The heterodimeric complex IrtAB has been identified as being responsible for the import of the two iron-loaded siderophores (Fe3+-MBT and Fe3+-cMBT) from the periplasmic space into the cytoplasm of Mtb and other mycobacteria. This protein complex is vital for the replication and viability of Mtb in macrophages, which reside in the lung alveoli. Like other ABC transporters, IrtAB contains two transmembrane domains (TMDs) and two nucleotide-binding domains (NBDs), with a single TMD and a single NBD in each of IrtA and IrtB. Interestingly, although IrtAB functions as an ABC importer, it adopts the canonical fold of type IV ABC exporters, which are normally responsible for the efflux of intracellular substrates such as the multidrug resistance protein, Sav1866.

To trap IrtAB in its ATP-bound state, the catalytic glutamate residues (Glu771 in IrtA and Glu495 in IrtB) were replaced by glutamine (IrtAB (E-Q)). By contrast, the SID-truncated IrtAB (E-Q) (IrtABΔSID (E-Q)) incubated with 10 mmol/L ATP-Mg2+ was suitable for cryo-EM and could be resolved at 3.1 Å resolution. Addition of ATP-Mg2+ resulted in an overall conformation that is substantially different from that of the ATP-free form. At the cytoplasmic side, the two NBDs of IrtA and IrtB form a “head-to-tail” dimer, characteristic of ABC transporters. Two ATP molecules are bound at the dimer interface, each of which is stabilized by an interaction between a Walker A motif in one NBD (IrtA or IrtB) and an ABC signature motif in the other NBD (IrtB or IrtA). Two magnesium ions are also observed, which ligand between the β- and γ-phosphates of ATP, a serine in the Walker A motif and the Q-loop glutamine, near the ABC signature motif. The TMHs of IrtAB do not split into two wings when ATP binds. As a result, the TMHs pack closely together to form an occluded amphipathic cavity with an approximate volume of ~4,600 Å3 (~2,700 Å3 in IrtA and ~1,900 Å3 in IrtB), which spans the entire thickness of the membrane and extends to the intracellular part of IrtAB. The marked difference between these two structures in the occluded state is that an additional unknown metal ion is observed in the cavity of IrtAB. However, the precise identity of the metal ion needs to be identified with more studies. This metal is bound to IrtA only and is liganded to three histidine residues (His356, His402, and His407), which are highly conserved across mycobacteria.

> MARGLQGVMLRSFGARDHTATVIETISIAPHFVRVRMVSPTLFQDAEAEPAAWLRFWFPDPNGSNTEFQRAYTISEADPAAGRFAVDVVLHDPAGPASSWARTVKPGATIAVMSLMGSSRFDVPEEQPAGYLLIGDSASIPGMNGIIETVPNDVPIEMYLEQHDDNDTLIPLAKHPRLRVRWVMRRDEKSLAEAIENRDWSDWYAWATPEAAALKCVRVRLRDEFGFPKSEIHAQAYWNAGRAMGTHRATEPAATEPEVGAAPQPESAVPAPARGSWRAQAASRLLAPLKLPLVLSGVLAALVTLAQLAPFVLLVELSRLLVSGAGAHRLFTVGFAAVGLLGTGALLAAALTLWLHVIDARFARALRLRLLSKLSRLPLGWFTSRGSGSIKKLVTDDTLALHYLVTHAVPDAVAAVVAPVGVLVYLFVVDWRVALVLFGPVLVYLTITSSLTIQSGPRIVQAQRWAEKMNGEAGSYLEGQPVIRVFGAASSSFRRRLDEYIGFLVAWQRPLAGKKTLMDLATRPATFLWLIAATGTLLVATHRMDPVNLLPFMFLGTTFGARLLGIAYGLGGLRTGLLAARHLQVTLDETELAVREHPREPLDGEAPATVVFDHVTFGYRPGVPVIQDVSLTLRPGTVTALVGPSGSGKSTLATLLARFHDVERGAIRVGGQDIRSLAADELYTRVGFVLQEAQLVHGTAAENIALAVPDAPAEQVQVAAREAQIHDRVLRLPDGYDTVLGANSGLSGGERQRLTIARAILGDTPVLILDQATAFADPESEYLVQQALNRLTRDRTVLVIAHRLHTITRADQIVVLDHGRIVERGTHEELLAAGGRYCRLWDTGQGSRVAVAAAQDGTR;> MIRTWIALVPNDHRARLIGFALLAFCSVVARAVGTVLLVPLMAALFGEAPQRAWLWLGWLSAATVAGWVLDAVTARIGIELGFAVLNHTQHDVADRLPVVRLDWFTAENTATARQAIAATGPELVGLVVNLVTPLTSAILLPAVIALALLPISWQLGVAALAGVPLLLGALWASAAFARRADTAADKANTALTERIIEFARTQQALRAARRVEPARSLVGNALASQHTATMRLLGMQIPGQLLFSIASQLALIVLAGTTAALTITGTLTVPEAIALIVVMVRYLEPFTAVSELAPALESTRATLGRIGSVLTAPVMVAGSGTWRDGAVVPRIEFDDVAFGYDGGSGPVLDGVSFCLQPGTTTAIVGPSGCGKSTILALIAGLHQPTRGRVLIDGTDVATLDARAQQAVCSVVFQHPYLFHGTIRDNVFAADPGASDDQFAQAVRLARVDELIARLPDGANTIVGEAGSALSGGERQRVSIARALLKAAPVLLVDQATSALDAENEAAVVDALAADPRSRTRVIVAHRLASIRHADRVLFVDDGRVVEDGSISELLTAGGRFSQFWRQQHEAAEWQILAE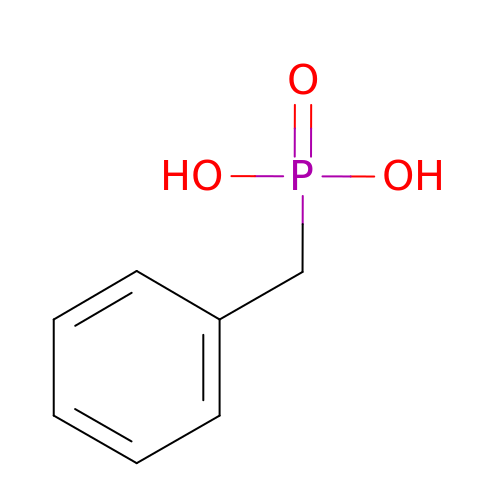benzylphosphonic acid | C7 H9 O3 P | OGBVRMYSNSKIEF-UHFFFAOYSA-N> AASELKQLETNNSPSTALGQISEGLTTLSHIPVLGNIF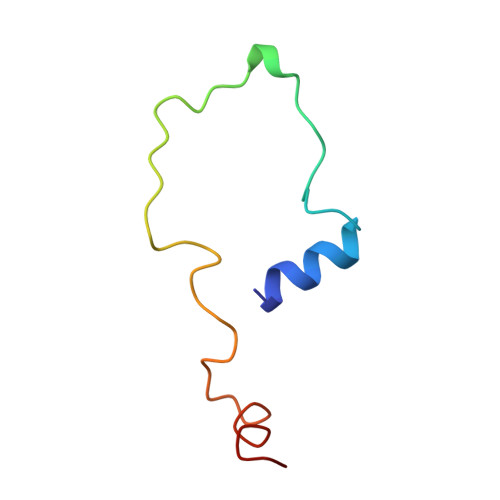STPAWISAKAADLAKLFGF> AGSGHMMELHILEHRVRVLSVARPGLWLYTHPLIKLLFLPRRSRCKFFSLTETPEDYTLMVDEEGFKELPPSEFLQVAEATWLVLNVSSHSGAAVQAAGVTKIARSVIAPLAEHHVSVLMLSTYQTDFILVREQDLSVVIHTLAQEFDIYREVGGEPVPVTRDDSSNGFPRTQHGPSPTVHPIQSPQNRFCVLTLDPETLPAIATTLIDVLFYSHSTPKEAASSSPEPSSITFFAFSLIEGYISIVMDAETQKKFPSDLLLTSSSGELWRM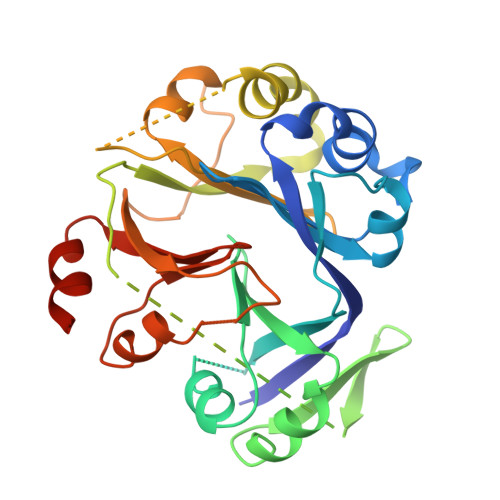VRIGGQPLGFDECGIVAQIIGPLAAADISAYYISTFNFDHALVPEDGIGSVIEVLQRRQEGLAS(3R,4S)-1-acetyl-4-phenylpyrrolidine-3-carboxylic acid | C13 H15 N O3 | 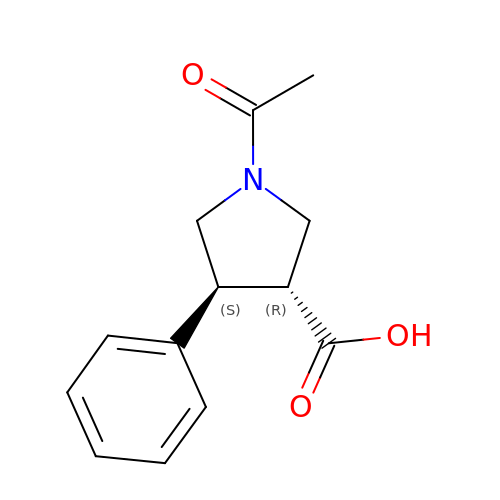UJHLINFGICYWPQ-NEPJUHHUSA-N> GGNSSTSALNSRRNSLDKSSN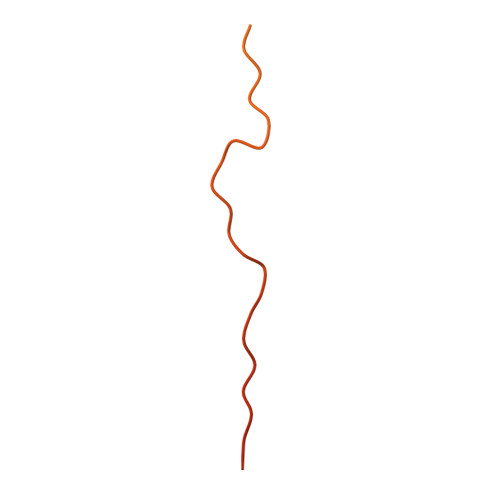KQGMSGLPPIFGGESTSYHHDNKIQKYNQLGVEEDDDDENDRLLNQMGNSATKFKSSISPRSIDSISSSFIKSRIPIRQPYHYSQPTTAPFQAQAKFHKPANKLIDNG>[2x]MTSALIERIDAIIVDLPTIRPHKLAMHTMQQQTLVVLRVRCSDGVEGIGEATTIGGLAYGYESPEGIKANIDAHLAPALIGLAADNINAAMLKLDKLAKGNTFAKSGIESALLDAQGKRLGLPVSELLGGRVRDSLEVAWTLASGDTARDIAEARHMLEIRRHRVFKLKIGANPVEQDLKHVVTIKRE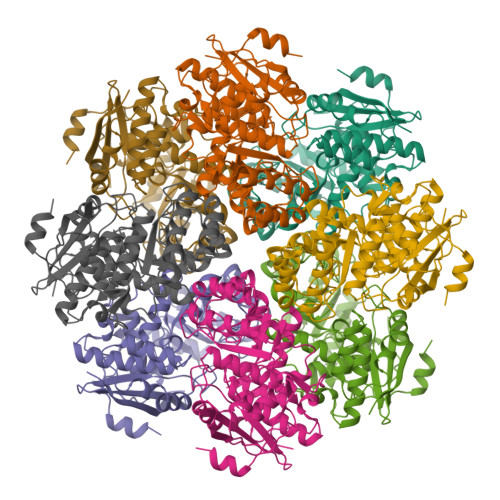LGDSASVRVDVNQYWDESQAIRACQVLGDNGIDLIEQPISRINRGGQVRLNQRTPAPIMADESIESVEDAFSLAADGAASIFALKIAKNGGPRAVLRTAQIAEAAGIGLYGGTMLEGSIGTLASAHAFLTLRQLTWGTELIGPLLLTEEIVNEPPQYRDFQLHIPRTPGLGLTLDEQRLARFARR>[13x]AESSGKSEAPPPAQTPEVGIVTLEAQTVTLNTELPGRTNAFRIAEVRPQVNGIILKRLFKEGSDVKAGQQLYQIDPATYEADYQSAQANLASTQEQAQRYKLLVADQAVSKQQYADANAAYLQSKAAVEQARINLRYTKVLSPISGR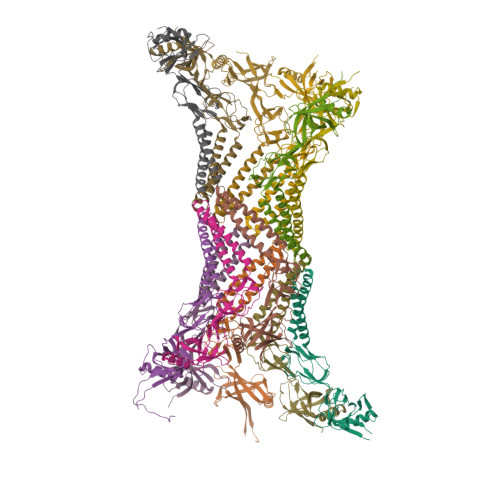IGRSAVTEGALVTNGQANAMATVQQLDPIYVDVTQPSTALLRLRRELASGQLERAGDNAAKVSLKLEDGSQYPLEGRLEFSEVSVDEGTGSVTIRAVFPNPNNELLPGMFVHAQLQEGVKQKAILAPQQGVTRDLKGQATALVVNAQNKVELRVIKADRVIGDKWLVTEGLNAGDKIITEGLQFVQPGVEVKTVPAKNVASAQKADAAPAKTDSKGHHHHHH> DSQWGSGKNLYDKVCGHCHKPEVGVGPVLEGRGLPEAYIKDIVRNGFRAMPAFPASYVDDESLTQVAEYLSSLPAPAA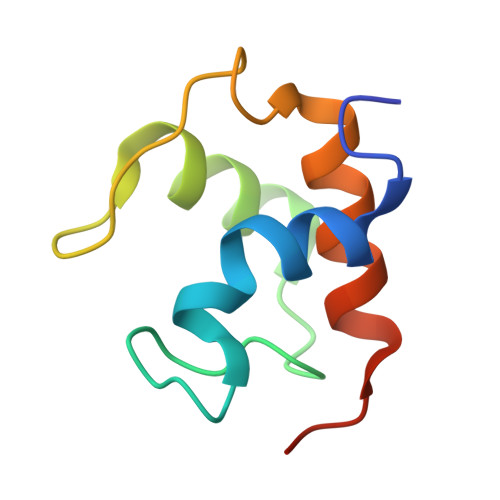QP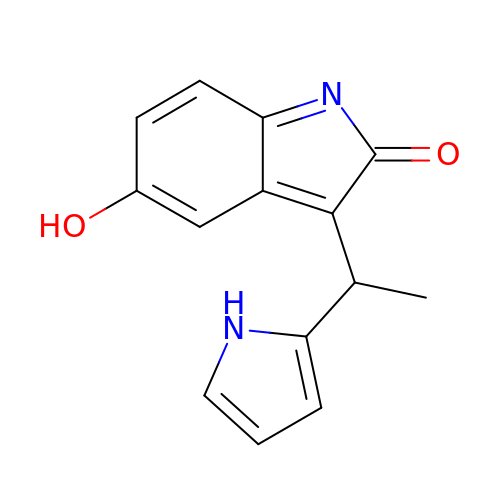5-HYDROXY-3-[(1R)-1-(1H-PYRROL-2-YL)ETHYL]-2H-INDOL-2-ONE | C14 H12 N2 O2 | VWQVBIPGKIAUGA-QMMMGPOBSA-N>[3x]MGDI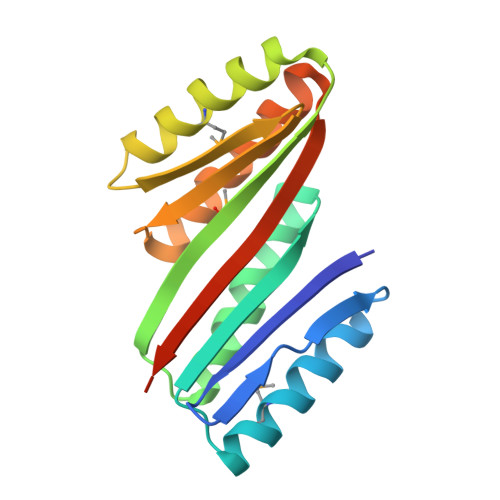QVQVNIDDNGKNFDYTYTVTTESELQKVLNELMDYIKKQGAKRVRISITARSSKEAYKFLAILAKVFAELGYNDINRKMTVRFRGDDLEALEKALKEMIRQARKFAGTVTYTLDGNDLEITITGVPRQVLEELAKEAERLAKEFNITITITVTVEGQLGSLEHHHHHH>MEFGSFLVSLGTSFVIFVILMLLFTWLSRKSGNAPIYYPNRILKGLEPWEGTSLTRNPFAWMREALTSSEQDVVNLSGVDTAVHFVFLSTVLGIFACSSLLLLPTLLPLAATDNNIKNTKNATDTTSKGTFSQLDNLSMANITKKSSRLWAFLGAVYWISLVTYFFLWKAYKHVSSLRAQALMSADVKPEQFAILVRDMPAPPDGQTQKEFIDSYFREIYPETFYRSLVATENSKVNKIWEKLEGYKKKLARAEAILAATNNRPTNKTGFCGLVGKQVDSIEYYTELINESVAKLETEQKAVLAEKQQTAAVVFFTTRVAAASAAQSLHCQMVDKWTVTEAPEPRQLLWQNLNIKLFSRIIRQYFIYFFVAVTILFYMIPIAFVSAITTLKNLQRIIPFIKPVVEITAIRTVLESFLPQIALIVFLAMLPKLLLFLSKAEGIPSQSHAIRAASGKYFYFSVFNVFIGVTLAGTLFNTVKDIAKNPKLDMIINLLATSLPKSATFFLTYVALKFFIGYGLELSRIIPLIIFHLKKKYLCKTEAEVKEAWYPGDL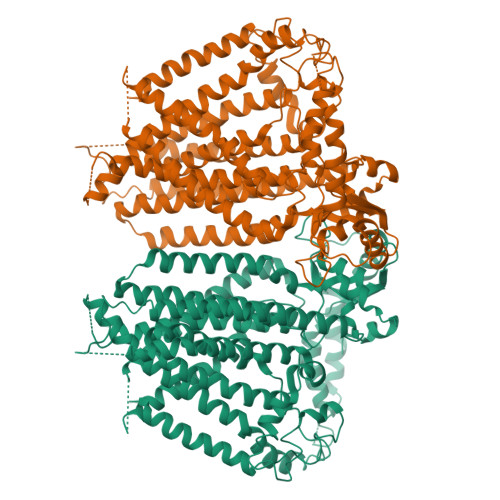SYATRVPGDMLILTITFCYSVIAPLILIFGITYFGLGWLVLRNQALKVYVPSYESYGRMWPHIHQRILAALFLFQVVMFGYLGAKTFFYTALVIPLIITSLIFGYVCRQKFYGGFEHTALEVACRELKQSPDLEEIFRAYIPHSLSSHKPEEHEFKGAMSRYQDFNAIAGV[2x]>[6x]AVANATELVNKISENCFEKCLTSPYATRNDACIDQCLAKYMRSWNVISKAYISRIQNASASGEI;>LEGENSKQKVQMSIHQFTNICFKKCVESVN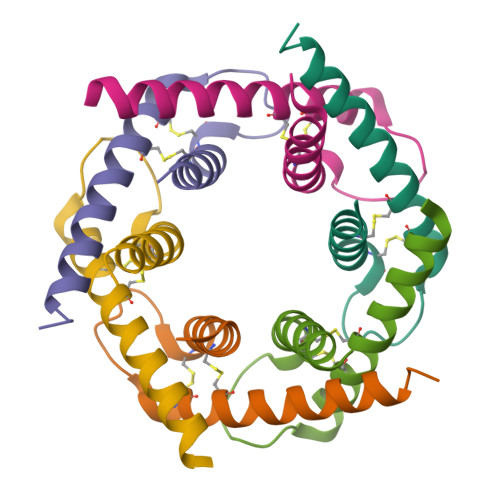DSNLSSQEEQCLSNCVNRFLDTNIRIVNGLQNTR[6x]> MATSGIVESFPTGALVPKAETGVLNFLQKYPEYDGRDVTIAIFDSGVDPRATGLETLCDGKTVKVIERYDCSGCGDVDMKKKVTPDENGNIKGLSGNSLKLSPELMALNTDPEKAVRVGLKSFSDLLPSKVRNNIVAQAKLKHWDKPHKTATANASRKIVEFESQNPGEASKLPWDKKILKENLDFELEMLNSYEKVYGDIKTSYDCILFPTADGWLTIVDTTEQGDLDQALRIGEYSRTHETRNVDDFLSISVNVHDEGNVLEVVGMSSPHGTHVSSIASGNHSSRDVDGVAPNAKIVSMTIGDGRLGSMETGTALVRAMTKVMELCRDGRRIDVINMSYGEHANWSNSGRIGELMNEVVNKYGVVWVASAGNHGPALCTVGTP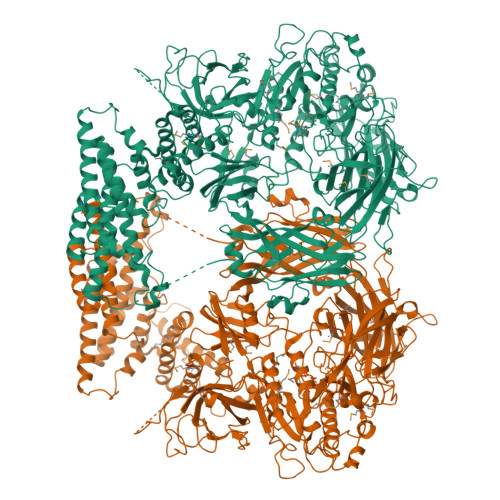PDISQPSLIGVGAYVSPQMMEAEYAMREKLPGNVYTWTSRDPCIDGGQGVTVCAPGGAIASVPQFTMSKSQLMNGTSMAAPHVAGAVALLISGLKQQNIEYSPYSIKRAISVTATKLGYVDPFAQGHGLLNVEKAFEHLTEHRQSKDNMLRFSVRVGNNADKGIHLRQGVQRNSIDYNVYIEPIFYNDKEADPKDKFNFNVRLNLIASQPWVQCGAFLDLSYGTRSIAVRVDPTGLQPGVHSAVIRAYDTDCVQKGSLFEIPVTVVQPHVLESDQNTPVFEPASSKGDNSVEFQPNTIQRDFILVPERATWAELRMRITDPNRGEDIGKFFVHTNQLLPKQSCRKLETMKIVSVGSENESIMAFKVKSGRILELCIAKYWSNYGQSHLKYSLRFRGVEAHNPNAYVMHAGRGIHKLEIEALVAEDVQPQLQLKNAEVVLKPTEAKISPLSATRDVIPDGRQVYQNLLAFNLNVAKAADVSIYAPIFNDLLYEAEFESQMWMLFDANKALVATGDAHSHTSFTKLDKGEYTIRLQVRHEKRDLLEKISEANLVASFKLTSPLTLDFYENYNQCIVGGRKYVSSPLRLSTRVLYIAPITQERLTKANLPAQCAWLSGNLVFPQDEVGRRVAQHPFTYILNPAEKKSHTNGSSNGSSAAGSTATAAAVTTANGAKPKAPATPQAATSVTNPAAGDGISVQNDPPVDSSGSPASPKKGKANADDYAESFRDFQCSQIVKCELEMAEKIYNDVVAAHPKHLQANLLLIQNIESNQLKSQLPLTFVNAQKTSPPEAGESADKQKEDQKKVRSALERIVKLADKVIQETDSEALLSYYGLKNDTRADAAKIKTNMDKQKNTLIEALSKKGIAVAKLAVLDDCIKDSLAEINELYTEIIKFVDANDSKAIQFALWHAYAHGHYGRMYKYVVKLIEEKRTRDHFVELAAINGALGHEHIRTVINRMMITAFPSSFRLF3-({4-hydroxy-1-[(2R)-2-methyl-3-phenylpropanoyl]piperidin-4-yl}methyl)quinazolin-4(3H)-one | C24 H27 N3 O3 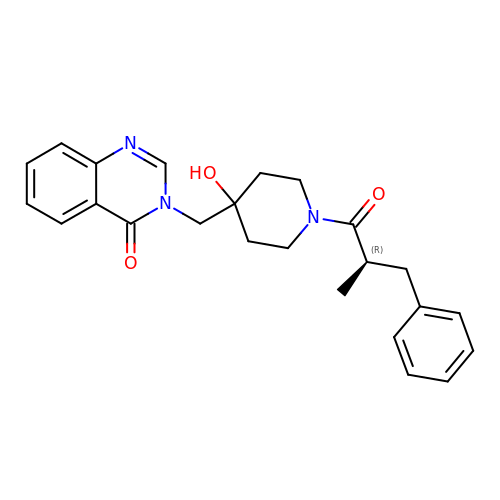| BAMWYPCZJUTPAE-GOSISDBHSA-N> MGSSHHHHHHMSGENLYFQGASSGKSVTSEHQTKDEMKTEQTASKTSAAKGKEVADFELMGVDGKTYRLSDYKGKKVYLKFWASWCSICLASLPDTDEIAKEAGDDYVVLTVVSPGHKGEQSEADFKNWYKGLDYKNLPVLVDPSGKLLETYGVRSYPTQAFIDKEGKLVKTHPGFMEKDAILQTLKELA

In addition, the molecular interplay of the surface-exposed TlpA (renamed Etrx1) with its extracellular paralogue Etrx2 on oxidative stress resistance and virulence are unknown. This study discovers the unique molecular architecture of two surface-exposed thioredoxin-systems, Etrx1 and Etrx2 and their redox partners CcdA1, CcdA2 and SpMsrAB2 as important pneumococcal extracellular reducing systems essential for pneumococcal pathogenesis and oxidative stress resistance. The bioinformatic analysis of pneumococcal genomes identified two genes encoding surface-exposed thioredoxin-like lipoproteins, renamed here Etrx1 and Etrx2. According to the accepted catalytic mechanism of thioredoxin-like proteins, Etrx1/Etrx2 would bind their redox partner SpMsrAB2 by means of a hydrophobic surface and subsequently perform a nucleophilic attack on the target disulphide bond via the N-terminal nucleophilic thiolate of the CXXC motif (Cys84 in Etrx1, Cys81 in Etrx2). Surface-exposed Etrx1 and Etrx2 deliver electrons to the SpMsrAB2 protein for the reduction of MsrA2 (by Etrx1 or Etrx2) and MsrB2 (by Etrx2) domains.

The Etrx1 model comprises amino acid residues from Ala53 to Leu187. Etrx1 presents a globular structure (38 × 28 × 29 Å) displaying a thioredoxin-like fold that contains seven β-strands and five α-helices. Besides the canonical Trx fold, Etrx1 has two insertions. The first insertion (residues 53–72) results in β1, β2 and α1 elements, and the second insertion (residues 112–144) gives rise to an additional β-strand (β5) and α-helix (α3). The loop connecting β3 with α2 contains the CXXC motif (84CSIC87) defining the nucleophilic active site Cys84 and the resolving Cys87. These cysteine residues form a disulphide bridge reflecting the oxidized state of the protein. The structural data clearly show that only the active site Cys84 is solvent-exposed and accessible for electron transfer reactions. At the beginning of the second insertion and near the active site there is an additional loop connecting β4 with α3 (residues 112–120) that is not present in the closely related family of cytochrome maturation proteins. Etrx1 lacks this cavity and this region shows differences in both the nature of the amino acids and in the conformation of the β4–α3 loop. In agreement with these results, soaking experiments with Etrx1 crystals did not yield a complex with Cyclofos-3™ even at high concentrations of the detergent.> AQTYEITYQNSFEGKINPNQNHIISITNSDKTLLFNEKIKNKKADFPFEVNEINRKNNEVSQFAFLNNNEIVKTSDNTILAKQEFKPTSETGKILGYNVKKAVTSVNSNTIEVWYTNDLKVKGGPSILGQDLGLVLKTVRNGSSVVEATSVKKIKALDDQSLFNGKNITEKDALTYKDMIWKSRFITIPVFENETINFSDASKSDQVIQRFGNGTIILKKVKIPEIKQGNTIFVELKQKSNGDAYDRTGDVFIIPQERAISYYTGLTQGVKSLPVYQNGNGKSYQGVALTPDYLPFIELMRFFTPFGIGHFNEKIQLKGKNWHNNTPYRQDITELRPQLSGKEILIGAFIGNYDKGGHQISLELSIHPDQQKIVNNNFVLPVFN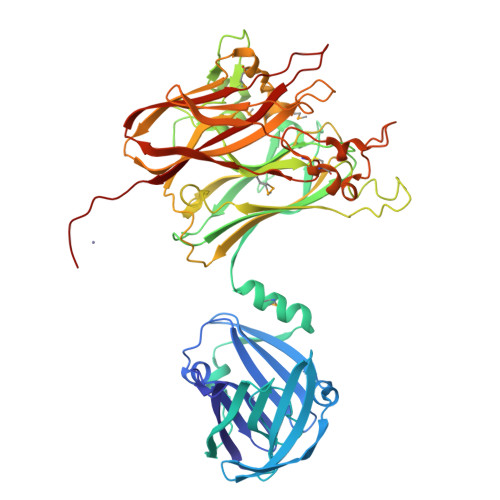TTNVMEMAGQDYPTMFNSDKGVEVDFILTKDLKNAQLRYITTGHGGWGAGDEFVPKENSIYLDGKLAHAFTPWRTDCGSYRLFNPASGNFEDGLSSSDLSRSNWCPGTITNPVYINLGNLNAGKHTIQVKIPQGAPEGSSQSFWNVSGVLLGQEHHHHHHHH>SENDSIELDDVANLMFYGEGQIGTNKQPFMFIFDTGSANLWVPSVNCDSIGCS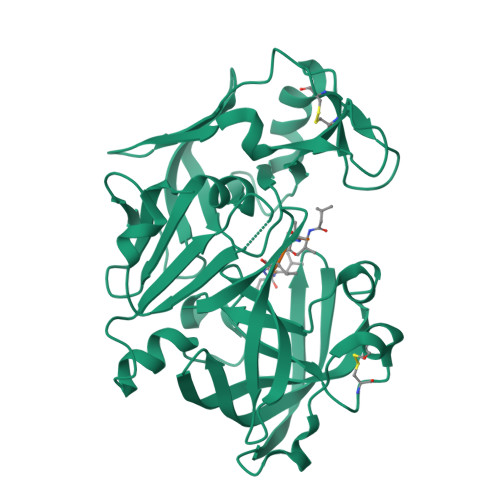TKHLYDASASKSYEKDGTKVEISYGSGTVRGYFSKDVISLGDLSLPYKFIEVTDADDLEPIYSGSEFDGILGLGWKDLSIGSIDPVVVELKKQNKIDNALFTFYLPVHDKHVGYLTIGGIESDFYEGPLTYEKLNHDLYWQIDLDIHFGKYVMQKANAVVDSGTSTITAPTSFLNKFFRDMNVIKVPFLPLYVTTCDNDDLPTLEFHSRNNKYTLEPEFYMDPLSDIDPALCMLYILPVDIDDNTFILGDPFMRKYFTVFDYEKESVGFAVAKNL[2x]>AGITGTWYNQLGSTFIVTAGADGALTGTYESAVGNAESRYVLTGRYDSAPATDGSGTALGWTVAWKNNYRNAHSATTWSGQYVGGAEARINTQWLLTSGTTEANAWKSTLV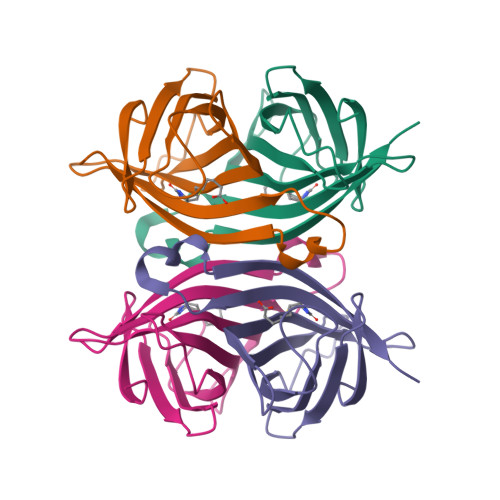GHDTFTKVKP[2x]XPB is a superfamily 2 (SF2) DNA helicase conserved from archaea to human. As the largest subunit of the transcription factor TFIIH complex, XPB is required for promoter melting in transcription and unwinding damaged DNA in nucleotide excision repair. In archaea, due to the lack of the TFIIH-like complex, XPB is in complex with Bax1, an XPG-like nuclease, to function as a helicase-nuclease machine for DNA unwinding and incision. Here, we report crystal structures of XPB from Sulfurisphaera tokodaii (St) bound to the nuclease Bax1 and their complex with a bubble DNA having one arm unwound in the crystal.

Extensive trials on crystallizing the full-length StXPB–Bax1 complex with DNA did not achieve diffracting quality crystals, so we engineered a truncated StBax1 by removing its C-terminal domain, which is absent in many archaeal Bax1 orthologues. The crystal structure of the StXPB–Bax1ΔC–DNA ternary complex was determined at 3.55 Å resolution (see Supplementary Table S1 for statistics of data collection and structure refinement). The DNA substrate used for the co-crystallization is a 24 base-pair (bp) DNA duplex containing a 6-nucleotide unpaired region (hereafter, bubble-6 DNA). Surprisingly, the 6-bp short arm of the bubble-6 DNA was unwound in the crystal, which is consistent with our previous observation that binding of XPB to DNA induces changes in DNA electrochemical properties even in the absence of ATP. The dsDNA region retains the B form while the two ssDNA tails are bent and split apart by XPB and Bax1ΔC, respectively. The DNA-bound StXPB-Bax1ΔC heterodimer spirally encircles the DNA substrate by the HD1/HD2/ThM of XPB and the NTD/CRD of Bax1, forming a tunnel for 10-bp DNA duplex binding with XPB closer to the fork. Furthermore, the ThM motif of XPB intrudes between the two ssDNA tails like a wedge with the 3′-overhang extending through the channel formed by the HD2/ThM of XPB and the 5′-overhang extending into the space between two N-terminal β-hairpins of Bax1ΔC. The interactions of XPB with the ds-ss DNA junction region are mainly mediated by residues from the RED and ThM motifs, two unique and important motifs among XPB homologues. When XPB translocates along the dsDNA ahead of the fork, the ThM motif grips the 3′ overhang tail and the tip of the ThM motif, particularly residue F278, functions as a wedge to break the base pairs along the way. In the ternary complex, Bax1ΔC interacts with the unpaired 5′-overhang nucleotides C13b, C15b, T16b and stabilizes the strand separation, likely enhancing the DNA unwinding by XPB. However, the nuclease domain of Bax1ΔC does not interact with DNA at all, suggesting that the nuclease activity is inhibited when the repair bubble is being created and extended by XPB helicase during DNA repair.

>[2x]GSVYLRYFKGLILSDAYAPGLKWSDELKAYSALAFKYRDVRKYFLEKEIEVEENVIDSLPFPLIKDKIELRDYQAEAVKAWLKEKRGIIVLPTGAGKTQVALKIVSIMKVATLIVVPTIDLITQWKERINKYLDFDPGIIGGGEDSLKGITVITYDSAYTRAEELGNKFPLLIFDEVHHLPSEGYSIMAQLFASPYRLGLTATPERDDGKHELYPILVGPIVYRKSVEELAGKYIAKYKIKKLYVSLTNEEKKRYDGLRKKLKDFLSSRGLKLQNLDDFHRLVKLAAKDKEAREALLAWHESLNIAVNSQSKIEKLREILQEYKNEKIIVFTRDTQMAYRISKTFLIPVVTYKTDKDEREEILQKFRDGEYRVIVASTVFDEGVDVPDATLAIVMGGYGTKRQFLQRLGRILRKKDKEALLIEIVTKGTADYRLSRRRRE;>MGLPWELARFSIVKDEVLPHFATNEDLDLANEIISLFKAGKKLGEIDEEIEYLEKIYDHKLVRAFVKLLTRLCEFELDSPIPPIQIRRELFKYGPVLDEKEREDIIQKVSKKLGADIMRFVFSDLDEEKKIIKAPTISAEDLIRWYNLSLLQTLLFKAYKLTVYVSSNWKEIIRRAKWLGLMYFAYDKPLRFEFLGPATLVKLTEKYGRNLAVLLQFIISSQNWKIEAELVLGKKFKRVYKLKLANFKELKELVIDEKRFDSSVEEKFYKDFTNVIKGWKIIREPEPLVVDNRVFIPDFLVEKGNLKVYVEIVGFWTKEYIKEKLDKLKKVKYPILILLNEELGKEKFNGMNVITYKRKIDISLVYKWLRELE[2x]>[2x]SKSTAEIRQAFLDFFHSKGHQVVASSSLVPHNDPTLLFTNAGMN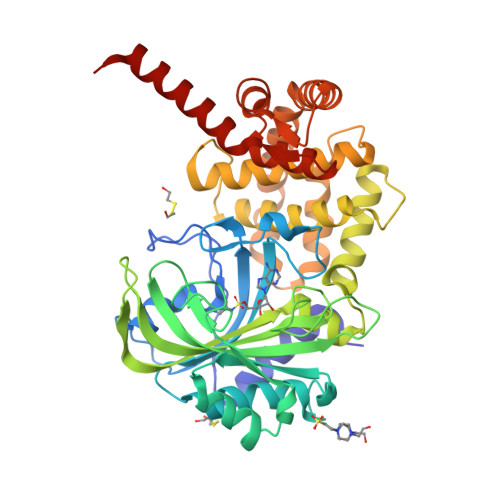QFKDVFLGLDKRNYSRATTSQRCVRAGGKHNDLENVGYTARHHTFFEMLGNFSFGDYFKLDAILFAWLLLTSEKWFALPKERLWVTVYESDDEAYEIWEKEVGIPRERIIRIGDNKGAPYASDNFWQMGDTGPCGPCTEIFYDHGDHIWGGPPGSPEEDGDRYIEIWNIVFMQFNRQADGTMEPLPKPSVDTAMGLERIAAVLQHVNSNYDIDLFRTLIQAVAKVTGATDLSNKSLRVIADHIRSCAFLIADGVMPSNENRGYVLRRIIRRAVRHGNMLGAKETFFYKLVGPLIDVMGSAGEDLKRQQAQVEQVLKTEEEQFARTLERGLALLDEELAKLSGDTLDGETAFRLYDTYGFPVDLTADVCRERNIKVDEAGFEAAMEEQRRRAREASGF6-[2-(3-fluoro-5-{2-[(2R,4S)-4-fluoropyrrolidin-2-yl]ethyl}phenyl)ethyl]-4-methylpyridin-2-amine 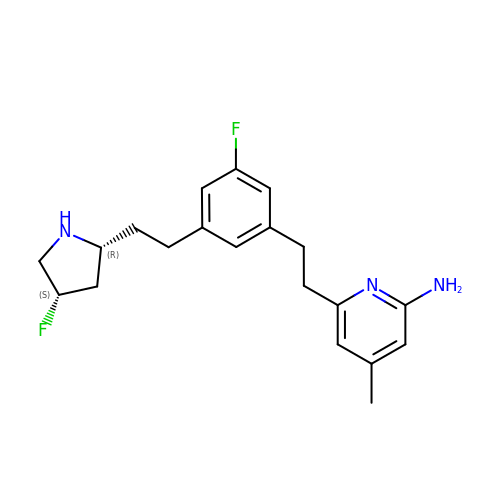| C20 H25 F2 N3 | PNHNZORGNQGMRR-ZWKOTPCHSA-N N-[4-cyano-3-(1H-1,2,4-triazol-5-yl)thiophen-2-yl]-2-(2-oxo-3,4-dihydroquinolin-1(2H)-yl)acetamide | C18 H14 N6 O2 S | 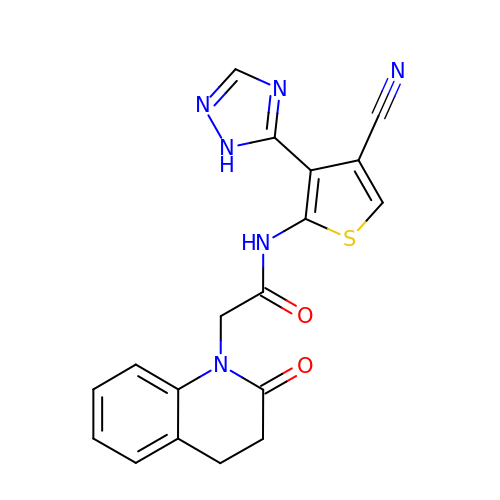WNRCGOJLZOLSJN-UHFFFAOYSA-N N-[4-(trifluoromethyloxy)phenyl]-1,3,4,9-tetrahydropyrido[3,4-b]indole-2-carbothioamide 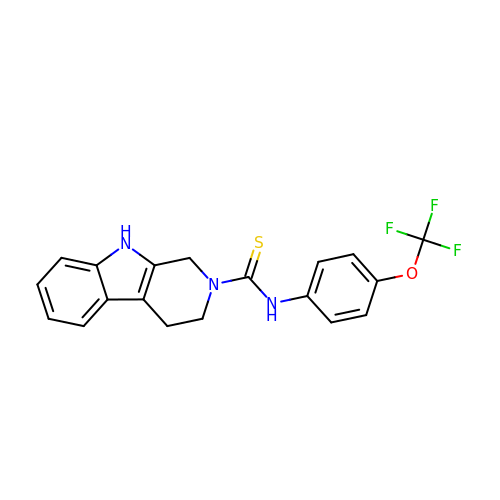| C19 H16 F3 N3 O S | CIBLQSZGHJTWDN-UHFFFAOYSA-N> DRVRNLQSEVEGVKNIMTQNVERILARGENLEHLRNKTEDLEATSEHFKTTSQKVARKFWWK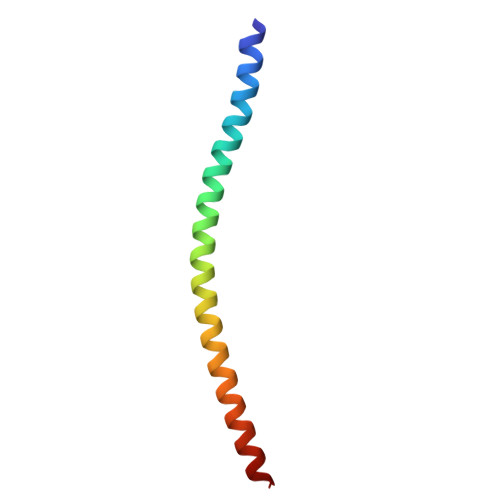NV Iron‐storage bacterioferritins (Bfrs), existing in either homo‐ or hetero‐multimeric form, play a crucial role in iron homeostasis. Unlike single‐subunit bacterial Ftn, Bfr can exist as a homo‐ or hetero‐complex, which assembles from two distinct subunits in a 1:1 ratio. The interior of the four‐helix bundle contains a ferroxidase center (FC), which catalyzes oxidation of Fe2+ to Fe3+. Here, the cryo‐EM structure and functional characterization of a bacterial hetero‐Bfr (SoBfr12) are reported.

By solving a 2.6 Å‐resolution cryo‐EM structure of SoBfr12, we found that although SoBfr12 adopts a conserved spherical cage‐like dodecahedron, its pores for ion entry, ferroxidase centers, and heme binding and iron reduction sites are significantly different from those of homo‐Bfrs. Differing from homo‐Bfrs, in which the subunits are arranged with O symmetry, the SoBfr12 near‐spherical nanocage comprises 12 SoBfr1 and 12 SoBfr2 subunits that are arranged in a C2 symmetry. During assembly, 12 subunits of the same type first form 6 homodimers, in which two subunits are arranged in an antiparallel direction, and no heterodimers were observed. Six heme‐free homodimers and six heme‐binding homodimers then assemble into a hetero‐Bfr nanocage in a fixed pattern. The most significant difference between SoBfr12 and homo‐Bfrs lies in that there is no heme bound at the interface of two SoBfr1 subunits because of the lack of the conserved heme binding residue (Met52), and as a result, SoBfr1 and SoBfr2 are unlikely to function equivalently. However, because all these pores are formed by two different homodimers in various combinations, the pores of the same type are not necessarily the same, resulting in 9 distinct subtypes: 4, 3, and 2 subtypes for B‐, 4‐fold, and 3‐fold pores, respectively. Remarkably, the interior surfaces of B‐pores, especially subtype I (3:0), are rich in negatively charged residues, and this feature likely facilitates the uptake of positively charged Fe2+ ions. Analysis of the surface electrostatic potential and hydrophobicity revealed that the subtype I 4‐fold pore formed by SoBfr1 only has a highly negative and hydrophilic pathway between the FC to the pore, along which Fe2+ ions move. Given that Glu94 plays a critical role in stabilizing two iron atoms, its substitution implies that the FCs of SoBfr2 may largely lose the ability to oxidize iron, and therefore SoBfr1 is primarily responsible for iron oxidation. All data from the cryo‐EM structure determination and biochemical and physiological analyses converge to support that hetero‐Bfrs are fundamentally different from homo‐Bfrs in structural details, including highly diverse pores, functionally differentiated FCs, and heme‐binding sites, which amount to substructures specialized for oxidation, mineralization, and reduction of iron ions.

>[12x]MKGDKDVIDALNRLLTGELSAMDQYFVHAHMYEDWGLNELYERIAHESDDEKGHAAKLVQRILFLEGVPNVAAREALNIGSNVEEMLRNDLAYEYKVADDLRKVIALCEQKKDYQTREILEVLLDDTESDHMYWLEKQLGLIDRIGLANYLQTKM;>MKGHPKVVGQLNRVLTCELTAINQYFLHARMFKHWGLEKLNHVEYKKSIEDMKHADKLIERVLFLEGLPNLQQLEKLRIGEHAQEMLDCDLAMVQEQLTLLRDAITLCEAEQDYVSRDLLEDILEDEEEHLDWLESQRELIGLTGIQNYLQSQISES[12x]N-(4-fluorophenyl)thiophene-2-carboxamide 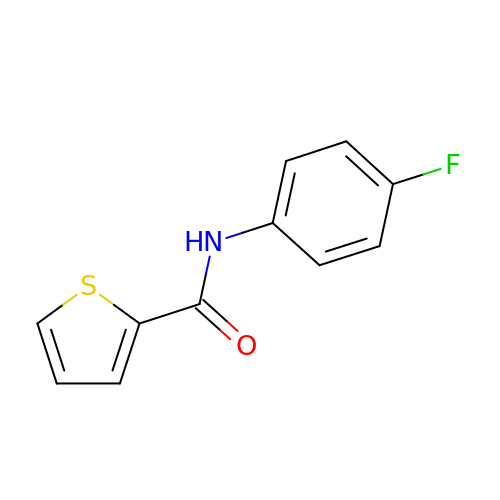| C11 H8 F N O S | GCPZKOCHNSMRNY-UHFFFAOYSA-N>[2x]GDRVKKLINSQISLLIGKGLHEFDSLRDPEVNDFRTKMRQFCEEAAAHRQQLGWVEWLQYSFPLQLEPSARGWRAGLLRVSNRALLVNVKFEGSEESFTFQVSTKDMPLALMACALRKKATVFRQPLVEQPEEYALQVNGRHEYLYGNYPLCHFQYICSCLHSGLTPHLTMVHSSSILAMRDEQSNPAPQVQKPRAKPPPIPAKKPSSVSLWSLEQPFSIELIEGRKVNADERMKLVVQAGLFHGNEMLCKTVSSSEVNVCSEPVWKQRLEFDIS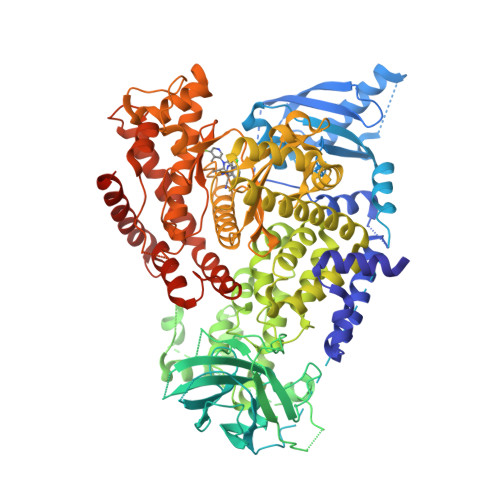VCDLPRMARLCFALYAVVEKAKKARSTKKKSKKADCPIAWANLMLFDYKDQLKTGERCLYMWPSVPDEKGELLNPAGTVRGNPNTESAAALVIYLPEVAPHPVYFPALEKILELGRHGERGRITEEEQLQLREILERRGSGELYEHEKDLVWKMRHEVQEHFPEALARLLLVTKWNKHEDVAQMLYLLCSWPELPVLSALELLDFSFPDCYVGSFAIKSLRKLTDDELFQYLLQLVQVLKYESYLDCELTKFLLGRALANRKIGHFLFWHLRSEMHVPSVALRFGLIMEAYCRGSTHHMKVLMKQGEALSKLKALNDFVKVSSQKTTKPQTKEMMHMCMRQETYMEALSHLQSPLDPSTLLEEVCVEQCTFMDSKMKPLWIMYSSEEAGSAGNVGIIFKNGDDLRQDMLTLQMIQLMDVLWKQEGLDLRMTPYGCLPTGDRTGLIEVVLHSDTIANIQLNKSNMAATAAFNKDALLNWLKSKNPGEALDRAIEEFTLSCAGYCVATYVLGIGDRHSDNIMIRESGQLFHIDFGHFLGNFKTKFGINRERVPFILTYDFVHVIQQGKTNNSEKFERFRGYCERAYTILRRHGLLFLHLFALMRAAGLPELSCSKDIQYLKDSLALGKTEEEALKHFRVKFNEALRESWKTKVNWLAHNVSKDNRQ4-[[N-[(PHENYLMETHOXY)CARBONYL]-/NL/N-LEUCYL]AMINO]-1[(2S)-2-[[[4-(PYRIDINYLMETHOXY)CARBONYL]AMINO]-4-METHYLPENT/NYL]-3-PYRROLIDINONE/N 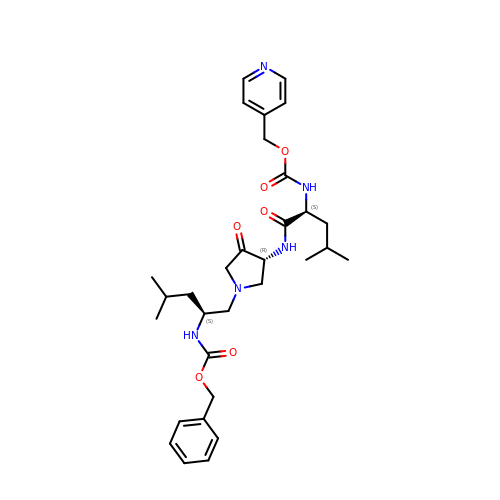| C31 H43 N5 O6 | YCGCXDDZHQMZQY-GMQQYTKMSA-N> GPIPTAPRENSLMFLSTTPDDTVPAYGNVRTPPVNYLPGEITDLLQLARIPTLMAFGRVPEPEPASDAYVPYVAVPTQFDDKPLISFPITLSDPVYQNTLVGAISSNFANYRGCIQITLTFCGPMMARGKFLLSYSPPNGTQPQTLSEAMQCTYSIWDIGLNSSWTFVIP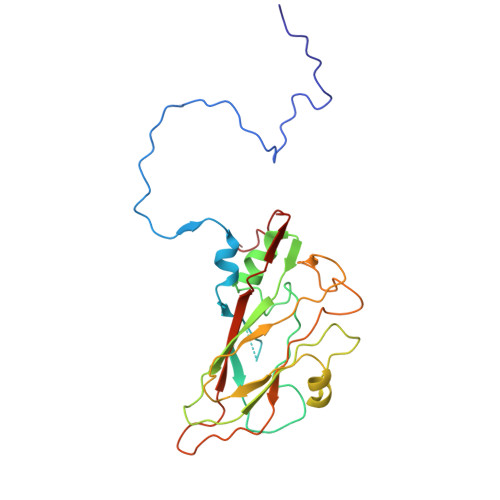YISPSDYRETRAITNSVYSADGWFSLHKLTKITLPPDCPQSPCILFFASAGEDYTLRLPVDCNPSYVF Here, we describe a rhodopsin group found in microorganisms from cold environments, such as glaciers, denoted as CryoRhodopsins (CryoRs). A distinguishing feature of the group is the presence of a buried arginine residue close to the cytoplasmic face. Combining single-particle cryo–electron microscopy and x-ray crystallography with rhodopsin activation by light, we demonstrate that the arginine stabilizes an ultraviolet (UV)–absorbing intermediate of an extremely slow CryoRhodopsin photocycle. Our data suggest that CryoRs are sensors for UV irradiation and are also capable of inward proton translocation modulated by UV light.

(A) Overall view of the CryoR1 pentamer in detergent micelles and nanodiscs. For the representation, the cryo-EM structure of CryoR1 at pH 8.0 was used. In contrast to all known MRs, there are no internal water molecules in the central region of CryoR1 and CryoR2. No densities in the maps and no space/internal cavities for waters were observed even at the cytoplasmic side of the retinal binding pocket, where normally at least one is found in other MRs near the highly conserved tryptophan residue of the helix F [W207/W208 in CryoR1/CryoR2 and W182 in BR (46, 47)]. In total, no water molecules were found in the radius of ~11 Å from the RSB, which is a unique feature of the studied CryoRs. At the extracellular side of CryoRs, we found a large water-filled cavity, between R99/R100 (in CryoR1/CryoR2; analog of R82 in BR) and the small (single turn) N-terminal α helix, capping the internal space of the CryoR protomer from the extracellular bulk. Aside from R99/R100, there are no internal rechargeable residues at the extracellular side of CryoRs. The exception is H230 in CryoR1, which is only found in 2 of 40 members of the CryoRs clade.

>[5x]MTDMISAPWEASLTQAEHSLIFYFLALTGSALLFGLARTWLTRGEVGARYRTAVVARSGIMIVATLSYVFMVLAFTSGYDHVGSLWVPNSEAIMTIAPRYVEWSIAVPLLSIELLSVATLSGVSARRTRLAAVAGAFLMIFTGFLGAVVIGDGRSVGSLIIWGAISTVFWIITAVILIRAIRHSLPQLTPEAAALLKTATIFLMSGWAVYPLAYLIQILFAGGLWTTSIHIILCTADIVVKLGFCGLIHRIAKLRTAEDVRAGVDIHTEAIWISSVKQSDAGIPTVVYLPEGETIHQRRPKPSDSNATASSSARQWTDDFPPTDL> MNILTDFRTHRPATLADAVNALAAEATLPLGAGTDLLPNLRRGLGHPAALVDLTGIDGLATISTLADGSLRIGAGATLEAIAEHDAIRTTWPALAQAAESVAGPTHRAAATLGGNLCQDTRCTFYNQSEWWRSGNGYCLKYKGDKCHVIVKSDRCYATYHGDVAPALMVLDARAEIVGPAGKRTVPVAQLFRESGAEHLTLEKGELLAAIEVPPTGAWSAAYSKVRIRDAVDFPLAGVAAA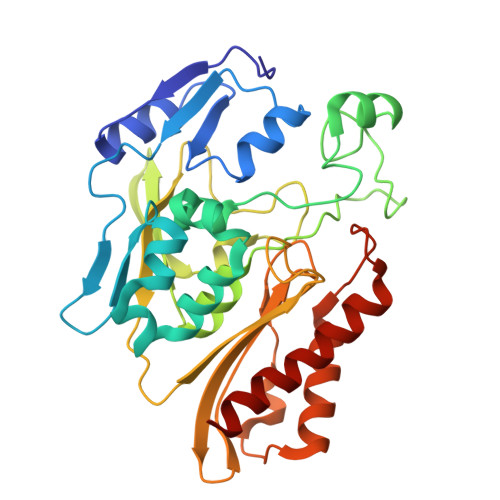LQRDGDRIAGLRVAITGSNSAPLMVPVDALLGGNWDDAAAETLAQLVRKTSNVLRTTITGVKYRRRVLLAISRKVVDQLWEAR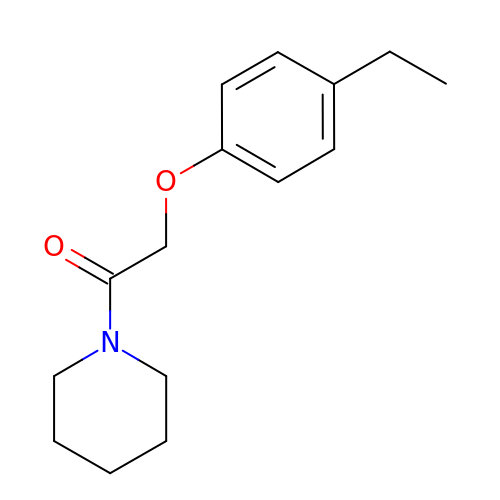2-(4-ethylphenoxy)-1-piperidin-1-yl-ethanone | C15 H21 N O2 | NWXWQKFUSIRDFR-UHFFFAOYSA-N>MSNLVLYTLHLSPPCRAVELTAKALGLELEQKTINLLTGDHLKPEFVKLNPQHTIPVLDDNGTIITESHAIMIYLVTKYGKDDSLYPKDPVKQARVNSALHFESGVLFARMRFIFERILFFGKSDIPEDRVEYVQKSYELLEDTLVDDFVAGPTMTIADFSCISTIS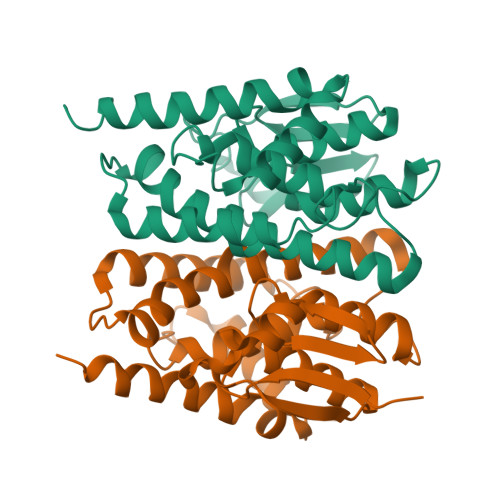SIMGVVPLEQSKHPRIYAWIDRLKQLPYYEEANGGGGTDLGKFVLAKKEENAKA[2x]>MLLEAIFHEAKGSYAYPISETQLRVRLRAKKGDVVRCEVLYADRYASPEEELAHALAGKAGSDERFDYFEALLECSTKRVKYVFLLTGPQGEAVYFGETGFSAERSKAGVFQYAYIHRSEVFTTPEWAKEAVIYQIFPERFANGDPSNDPPGTEQWAKDARPRHDSFYGGDLKGVIDRLPYLEELGVTALYFTPIFASPSHHKYDTADYLAIDPQFGDLPTFRRLVDEAHRRGIKIILDAVFNHAGDQFFAFRDVLQKGEQSRYKDWFFIEDFPVSKTSRTNYETAAVQVPAMPKLRTENPEVKEYLFDVARFWMEQGIDGWRLDVANEVDHAFWREFRRLVKSLNPDALIVGEIWHDASGWLMGDQFDSVMNYLFRESVIRFFATGEIHAERFDAELTRARMLYPEQAAQGLWNLLDSHDTERFLTSCGGNEAKFRLAVLFQMTYLGTPLIYYGDEIGMAGATDPDCRRPMIWEEKEQNRGLFEFYKELIRLRHRLASLTRGNVRSWHADKQANLYAFVRTVQDQHVGVVLNNRGEKQTVLLQVPESGGKTWLDCLTGEEVHGKQGQLKLTLRPYQGMILWN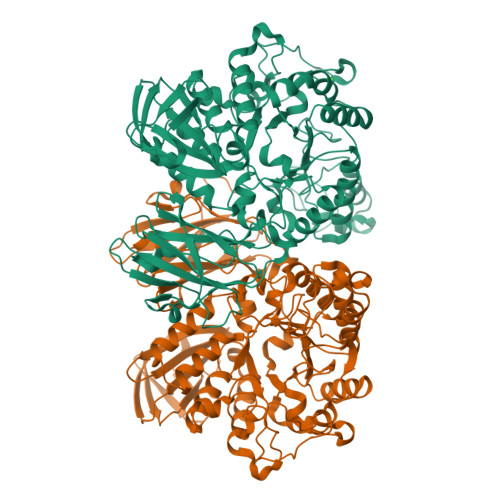GR[2x]>[6x]MSLQLLRNTRIFVSTVKTGHNKTNTQEILVQDDISWGQDSNSTDITVNEAGPRPTRGSKRFNDSLNAAEWSFSTYILPYKDKNTSKQIVPDYMLWHALSSGRAINLEGTTGAHNNATNFMVNFKDNSYHELAMLHIYILTDKTWSYIDSCQINQAEVNVDIEDIGRVTWSGNGNQLIPLDEQPFDPDQIGIDDETYMTIQGSYIKNKLTILKIKDMDTNKSYDIPITGGTFTINNNITYLTPNVMSRVTIPIGSFTGAFELTGSLTAYLNDKSLGSMELYKDLIKTLKVVNRFEIALVLGGEYDDERPAAILVAKQAHVNIPTIETDDVLGTSVEFKAIPSDLDAGDEGYLGFSSKYTRTTINNLIVNGDGATDAVTAITVKSAGNVTTLNRSATLQMSVEVTPSSARNKEVTWAITAGDAATINATGLLRADASKTGAVTVEATAKDGSGVKGTKVITVTAGG;>[3x]MFYSLMRESKIVIEYDGRGYHFDALSNYDASTSFQEFKTLRRTIHNRTNYADSIINAQDPSSISLAINFSTTLIESNFFDWMGFTREGNSLFLPRNTPNIEPIMFNMYIINHNNSCIYFENCYVSTVDFSLDKSIPILNVGIESGKFSEVSTFRDGYTITQGEVLPY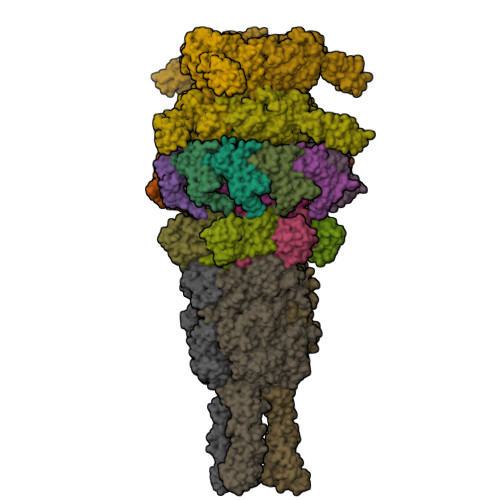SAPAVYTNSSPLPALISASMSFQQQCSWREDRNIFDINKIYTNKRAYVNEMNASATLAFYYVKRLVGDKFLNLDPETRTPLIIKNKYVSITFPLARISKRLNFSDLYQVEYDVIPTADSDPVEINFFGERK;>[12x]MSTENRVIDLVVDENVPYGLLMQFMDVDDSVYPSTSKPVDLTDFSLRGSIKSSLEDGAETVASFTTAIVDAAQGVASISLPVSAVTTIASKASKERDRYNPRQRLAGYYDVIITRTAVGSAASSFRIMEGKVYISDGVTQ;>[6x]MRLPDPYTNPEYPGLGFESVNLVDNDPMIRDELPNGKVKEVKISAQYWGINISYPELFPDEYAFLDSRLLEYKRTGDYLDVLLPQYEAFRVRGDTKSVTIPAGQKGSQIILNTNGTLTGQPKAGDLFKLSTHPKVYKITNFSSSGNVWNISLYPDLFITTTGSEKPVFNGILFRTKLMNGDSFGSTLNNNGTYSGISLSLRESL;>[3x]MKKILDSAKNYLNTHDKLKTACLIALELPSSSGSAATYIYLTDYFRDVTYNGILYRSGKVKSISSHKQNRQLSIGSLSFTITGTAEDEVLKLVQNGVSFLDRGITIHQAIINEEGNILPVDPDTDGPLLFFRGRITGGGIKDNVNTSGIGTSVITWNCSNQFYDFDRVNGRYTDDASHRGLEVVNGTLQPSNGAKRPEYQEDYGFFHSNKSTTILAKYQVKEERYKLQSKKKLFGLSRSYSLKKYYETVTKEVDLDFNLAAKFIPVVYGVQKIPGIPIFADTELNNPNIVYVVYAFAEGEIDGFLDFYIGDSPMICFDETDSDTRTCFGRKKIVGDTMHRLAAGTSTSQPSVHGQEYKYNDGNGDIRIWTFHGKPDQTAAQVLVDIAKKKGFYLQNQNGNGPEYWDSRYKLLDTAYAIVRFTINENRTEIPEISAEVQGKKVKVYNSDGTIKADKTSLNGIWQLMDYLTSDRYGADITLDQFPLQKVISEAKILDIIDESYQTSWQPYWRYVGWNDPLSENRQIVQLNTILDTSESVFKNVQGILESFGGAINNLSGEYRITVEKYSTNPLRINFLDTYGDLDLSDTTGRNKFNSVQASLVDPALSWKTNSITFYNSKFKEQDKGLDKKLQLSFANITNYYTARSYADRELKKSRYSRTLSFSVPYKFIGIEPNDPIAFTYERYGWKDKFFLVDEVENTRDGKINLVLQEYGEDVFINSEQVDNSGNDIPDISNNVLPPRDFKYTPTPGGVVGAIGKNGELSWLPSLTNNVVYYSIAHSGHVNPYIVQQLENNPNERMIQEIIGEPAGLAIFELRAVDINGRRSSPVTLSVDLNSAKNLSVVSNFRVVNTASGDVTEFVGPDVKLAWDKIPEEEIIPEIYYTLEIYDSQDRMLRSVRIEDVYTYDYLLTYNKADFALLNSGALGINRKLRFRIRAEGENGEQSVGWATI;>[3x]MTDKLIRELLIDVKQKGATRTAKSIENVSDALENAAAASELTNEQLGKMPRTLYSIERAADRAAKSLTKMQASRGMAGITKSIDGIGDKLDYLAIQLIEVTDKLEIGFDGVSRSVKAMGNDVAAATEKVQDRLYDTNRALGGTSKGFNDTAGAAGRASRALGNTSGSARGATRDFAAMAKIGGRLPIMYAALASNVFVLQTAFESLKVGDQLNRLEQFGTIVGTMTGTPVQTLALSLQNATNGAISFEEAMRQASSASAYGFDSEQLEQFGLVARRAAAVLGVDMTDALNRVIKGVSKQEIELLDELGVTIRLNDAYENYVKQLNATSTGIKYTVDSLTTYQKQQAYANEVIAESTRRFGYLDDALKATSWEQFAANANSALRSLQQSAATYLNPVMDTLNTFLYQTKSSQMRVSAMARSASAKTTPAENVTALIENAVGAREDLDTYLKESEERVKKAQELKQQLDDLKAKQAATAPIANALTAGGIGGDESNKLVVQLTNELARQNKEIEERTKTEKVLRQAVQDTGEALLRNGKLAEQLGAKMKYADTAVPGDKGVFEVDPNNLKAVSEIQKNFDFLKKSSSDTANNIRMAASSITNAKKASSDLNSVVKAVEDTSKVTGQSADTLVKNLNLGFSSLDQMKAAQKGLSEYVTAMDKSEQNALEVAKRKDEVYNQTKDKAKAEAAAREVLLRQQQEQLTAAKALLAINPNDPEALKQVAKIETEILNTKAQGFENAKKTKDYTDKILGVDREIALLNDRTMTSTQYRLAQLRLELQLEQEKTELYSKQADGQAKVEQSRRAQAQISREIWEAEKQGTASHVSALMDALEVSQTQRNVTGQSQILTERLSILQQQLELSKGNTEEELKYRNEIYKTSAALEQLKKQRESQMQQQVGSSVGATYTSTTGLIGEDKDFADMQNRMASYDQAISKLSELNSEATAVAQSMGNLTNAMIQFSQGSLDTTSMIASGMQTVASMIQYSTSQQVSAIDQAIAAEQKRDGKSEASKAKLKKLEAEKLKIQQDAAKKQIIIQTAVAVMQAATAVPYPFSIPLMVAAGLAGALALAQASSASGMSSIADSGADTTQYLTLGERQKNVDVSMQASSGELSYLRGDKGIGNANSFVPRAEGGMMYPGVSYQMGEHGTEVVTPMVPMKATPNDQLSDGSKTTSGRPIILNISTMDAASFRDFASNNSTAFRDAVELALNENGTTLKSLGNS> GSHMGQELVSLEGHQSAITALAFSKNIVVSGAADGTIKVWDILTGQLLRDHDGHQSEVTALQFKDNIVVSGAKDGTVKVWYIGTGQELVSLEGHQSAITALAFSKNIVVSGAADGTIKVWDILTGQLLRDHDGHQSEVTALQFKDNIVVSGAKDGTVKVWYIGTGQELVSLEGHQSAITALAFSKNIVVSGAADGTIKVWDILTGQLLRDHDGHQSEVTALQFKDNIVVSGAKDGTVKVWYIGTGQELVSLEGHQSAITALAFSKNIVVSGAADGTIKVWDILTGQLLRDHDGHQSEVTALQFKDNIVVSGAKDGTVKVWYIGT

WD40 proteins are a subfamily of propeller proteins with no intrinsic enzymatic activity, but their stable, modular architecture and versatile surface have allowed evolution to adapt them to many vital roles. By computationally reverse-engineering the duplication, fusion and diversification events in the evolutionary history of a WD40 protein, a perfectly symmetrical homologue called Tako8 was made. A different computational approach was employed to redesign Tako8 to create Ika8, a fourfold-symmetrical protein in which neighbouring blades carry compensating charges. Tako and Ika are the first successfully designed eight-bladed WD40-repeat proteins for which structures have been confirmed crystallographically.

The concentration of negatively charged residues reflects their high conservation in the parental template structures, so Ika8 was designed as a fourfold-symmetrical protein, allowing the search algorithm to identify compensating interactions between adjacent blades. Ika8 produced two crystal forms in space group P63, with one or three copies in the asymmetric unit. In one crystal form of Ika8 this axis is crystallographic, but in the other (and in the Ika4 crystals) it is noncrystallographic. In all crystal forms, the Ika proteins assemble as trimers which stack on top of each other into pillars. Unlike in the Tako8 protein, the conserved inter­actions stabilizing the crystal assembly involve hydrogen bonds between the outer rims of neighbouring molecules, while the interactions at the top face are mediated by water molecules and are not conserved. In comparison, only the alternating repeats of the Ika proteins can be superposed, in contrast to the template structure where the overlap of the individual blades is much poorer. The symmetry is also visible in the electrostatic potential map, where eightfold and fourfold symmetry can be observed for Tako8 and Ika8, respectively, with the exception of small differences owing to crystal-packing inter­actions; such charge symmetry is absent from the template protein. The melting/denaturation curves show that the Ika proteins are more stable than Tako8, especially under low-salt conditions.> MSTAKAPTLPASIFRAYDIRGVVGDT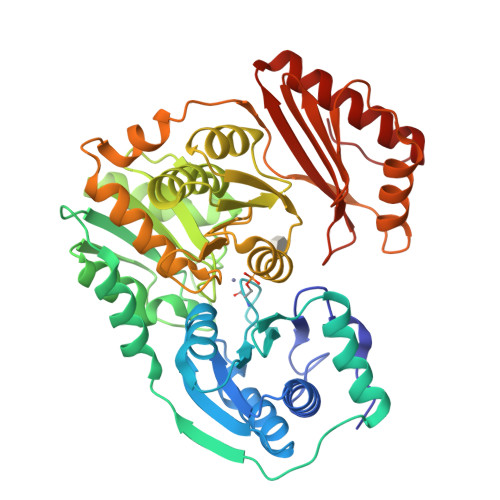LTAETAYWIGRAIGSESLARGEPCVAVGRDGRLSGPELVKQLIQGLVDCGCQVSDVGMVPTPVLYYAANVLEGKSGVMLTGSHNPPDYNGFKIVVAGETLANEQIQALRERIEKNDLASGVGSVEQVDILPRYFKQIRDDIAMAKPMKVVVDCGNGVAGVIAPQLIEALGCSVIPLYCEVDGNFPNHHPDPGKPENLKDLIAKVKAENADLGLAFDGDGDRVGVVTNTGTIIYPDRLLMLFAKDVVSRNPGADIIFDVKCTRRLIALISGYGGRPVMWKTGHSLIKKKMKETGALLAGEMSGHVFFKERWFGFDDGIYSAARLLEILSQDQRDSEHVFSAFGSDISTPEINITVTEDSKFAIIEALQRDAQWGEGNITTLDGVRVDYPKGWGLVRASNTTPVLVLRFEADTEEELERIKTVFRNQLKAVDSSLPVPF> ADPKETCSTGLYTHSGECCKACNLGEGVAQPCGADQTVCEPCLDSVTFSDVVSATEPCKPCTECLGLQSMSAPCVEADDAVCRCAYGYYQDEETGHCEACSVCEVGSGLVFSCQDKQNTVCEECPEGTYSDEANHVDPCLPCTVCEDTERQLRECTPWA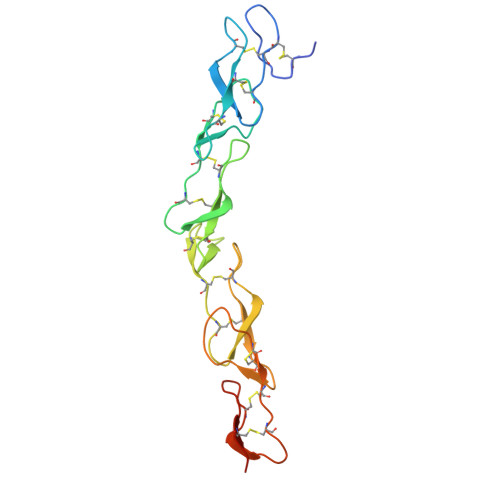DAECEHHHHHHH> MSLRIDVDTNFPECVVDAGKVTLGTQQRQEMDPRLREKQNEIILRAVCALLNSGGGIIKAEIENKGYNYERHGVGLDVPPIFRSHLDKMQKENHFLIFVKSWNTEAGVPLATLCSNLYHRERTSTDVMDSQEALAFLKCRTQTPTNINVSNSLGPQAAQGSVQYEGNINVSAAALFDRKRLQYLEKLNLPESTHVEFVMFSTDVSHCVKDRLPKCVSAFANTEGGYVFFGVHDETCQVIG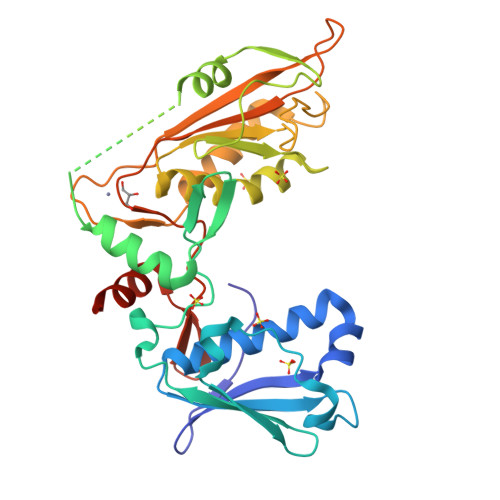CEKEKIDLTSLRASIDGCIKKLPVHHFCTQRPEIKYVLNFLEVHDKGALRGYVCAIKVEKFCCAVFAKVPSSWQVKDNRVRQLPTREWTAWMMEADLEHHHHHH>[3x]MASDGYTIKPNKKVTYSALGEDERMIGFSYKDFGISSSEKITEVQVNIS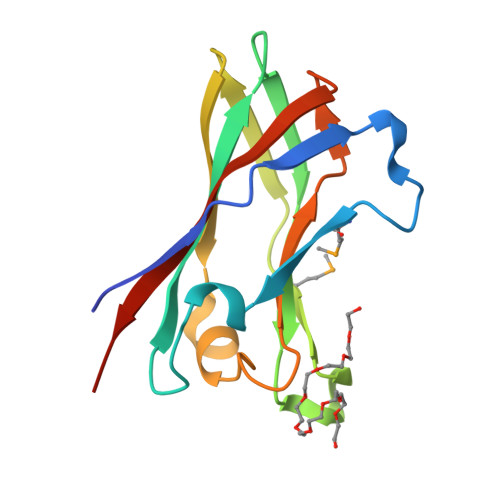ANKNIGKYVGQFGTSTTDSANGYWAMGDEITQSISGNSGTITWKVPSDISSIIQTQYGGEIKFGVWWIDCDEFTIDSVVLKLEHHHHHH> MAETLEKKHERIMLRFDRAYSPQKEVREKCIEATRFARVPGGQWEGATAAGTKLDEQFEKYPKFEINKVATELNRIIAEYRNNRITVKFRPGDREASEELANKLNGLFRADYEETDGGEACDNAFDDAATGGFGCFRLTSMLVNEYDPMDDRQRIAIEPIYDPSRSVWFDPDAKKYDKSDALWAFCMYSLSPEKYEAEYGKKPP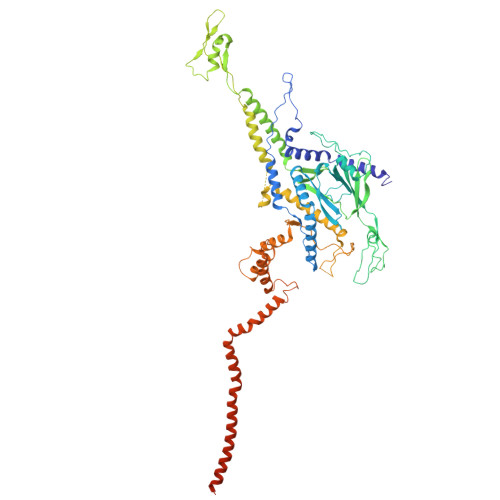TSLDVTSMTSWEYNWFGADVIYIAKYYEVRKESVDVISYRHPITGEIATYDSDQVEDIEDELAIAGFHEVARRSVKRRRVYVSVVDGDGFLEKPRRIPGEHIPLIPVYGKRWFIDDIERVEGHIAKAMDPQRLYNLQVSMLADTAAQDPGQIPIVGMEQIRGLEKHWEARNKKRPAFLPLREVRDKSGNIIAGATPAGYTQPAVMNQALAALLQQTSADIQEVTGGSQAMQQMPSNIAQETVNNLMNRADMASFIYLDNMAKSLKRAGEVWLSMAREVYGSEREVRIVNEDGSDDIAVLSAQVVDRQTGAVVALNDLSVGRYDVTVDVGPSYTARRDATVSVLTNVLSSMLPTDPMRPAIQGIILDNIDGEGLDDFKEYNRNQLLISGIAKPRNEKEQQIVQQAQMAAQSQPNPEMVLAQAQMVAAQAEAQKATNETAQTQIKAFTAQQDAMESQANTVYKLAQARNIDDKAVMEAIRLLKDVAESQQQQFQSPPQSPADLMPS>[2x]MVATPVKQKYDIKDISLAPQGRQRIEWAAREMPVLKQIRERFAQEKPFAGIRLVACCHVTTETANLAIALHAGGADSLLIASNPLSTQDDVAACLVADYGIPVYAIKGEDNETYHRHVQIALDHRPNIIIDDGSDVVATLVQERQHQLSDIIGTTEETTTGIVRLRAMFNDGVLTFPAMNVNDADTKHFYDNRYGT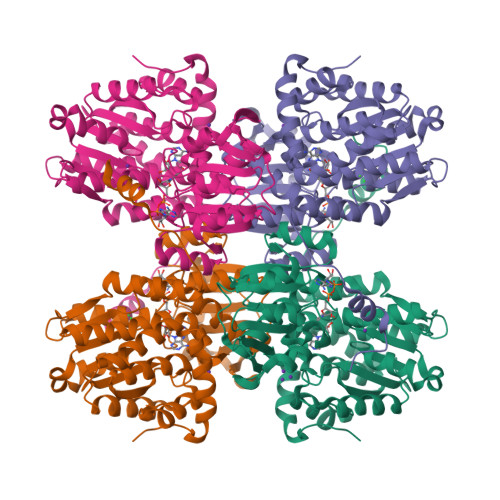GQSTLDGIIRATNILLAGKTIVVAGYGWCGKGVAMRAKGMGADVIVTEISPVPAIEAAMDGFRVMPMAEAAHQGDIFITVTGNKHVIRPEHFAVMKDGAIVCNSGHFDIEIDLKSLKEQAKEVKEVRNFTEQYILPNGKSIIVIGEGRLVNLAAAEGHPSAVMDMSFANQALACEHLVKNKGQLEPGMHSIPVEVDQEIARLKLQAMGIAIDSLTPEQVEYINSWASGT8-(4-beta-D-glucopyranuronosylpiperazin-1-yl)-5-(methylamino)-1,2,3,4-tetrahydro[1,2,3]triazino[4',5':4,5]thieno[2,3-c]isoquinoline | C23 H29 N7 O6 S | 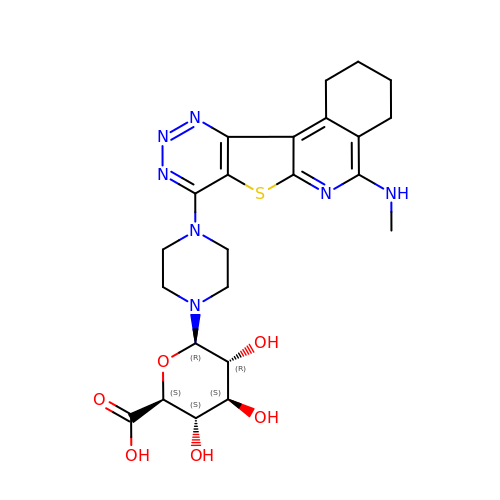DSFGEPIJIZKUTO-YSVRDODPSA-N> MGSHHHHHHMGQSVEVEILLNDAESRKRAEHKTEDGKKEKYFLFYDGETVSGKVSLSLKNPNKRLEHQGIKIEFIGQIELYYDRGNHHEFVSLVKDLARPGEITQSQAFDFEFTHVEKPYESYTGQNVKLRYFLRATISRRLNDVVKEM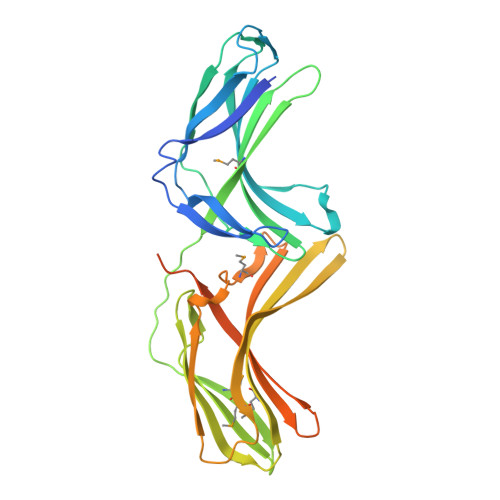DIVVHTLSTYPELNSSIKMEVGIEDCLHIEFEYNKSKYHLKDVIVGKIYFLLVRIKIKHMEIDIIKRETTGTGPNVYHENDTIAKYEIMDGAPVRGESIPIRLFLAGYELTPTMRDINKKFSVRYYLNLVLIDEEERRYFKQQEVVLWRKGDIVRKSMSHQAAIASQRFEGTTSLGEVRTPGQLSDNNSRQ5-[(1R,2S,4R,6R,7R,10S,11S,14S,16R)-14-hydroxy-7,11-dimethyl-3-oxapentacyclo[8.8.0.02,4.02,7.011,16]octadecan-6-yl]pyran-2-one | C24 H32 O4 | 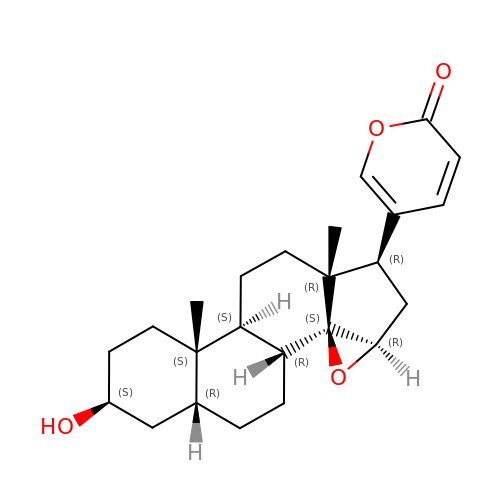ATLJNLYIJOCWJE-CWMZOUAVSA-N The SspH/IpaH family of novel E3 ligases are found in a number of Gram-negative bacteria and are used to target host enzymes for degradation to support pathogenesis. NELs are found in a number of Gram-negative bacteria, such as the mammalian pathogens Salmonella and Shigella and plant pathogens Ensifer fredii and Ralstonia solanacearum. They are composed of an N-terminal secretion motif, a leucine-rich repeat (LRR) domain, and a C-terminal NEL catalytic domain and are structurally conserved across the family. Crystal structures and mechanistic studies of NELs have provided insight into the activities of the two key functional domains: the LRR domain, which is responsible for substrate recognition, and the NEL domain, which can be divided into two subdomains: the C-terminal subdomain containing the E2–Ub binding domain (E2–UbBD) “thumb" and the N-terminal subdomain, which encompasses the catalytic E3 region containing the active site cysteine. Many pathogenic bacteria contain E3 ligases, most of which structurally resemble their eukaryotic counterparts, yet some bacteria, including Salmonella and Shigella, have evolved a new class of E3 ligases, the novel E3 ligase (NEL) family, that have no structural homology to eukaryotic E3s in their catalytic domain but function via an active site cysteine, analogous to HECT or RBR E3 ligases. These catalytic cysteine-containing E3 ligases transfer Ub onto the substrate in a two-step reaction: first, Ub is transferred from the E2–Ub conjugate to form an E3–Ub conjugate in a transthiolation reaction, and subsequently onto lysine residues in the substrate or Ub itself via an aminolysis reaction.

To better understand the mechanism of SspH1 and the apparent differences in activity, we solved the crystal structure of a construct containing the LRR and NEL domains but lacking the first 160 residues, ΔNSspH1 (now referred to as SspH1). The structure was refined at 2.9 Å resolution with one copy in the asymmetric unit and a P622 space group. The structure is elongated with the LRR (residues 161–393) domain extending away from the NEL domain (residues 405–622), which contains the catalytic cysteine (C492) and the α-helices of the E2–UbBD (residues 623–697). It is similar to IpaH9.8 and IpaH3 in an “open" conformation, with the position of the E2–UbBD relative to the catalytic loop in an analogous position to other bacterial E3 ligase structures. The E2–UbBD of SspH1 consists of two long antiparallel α-helices and a small C-terminal helical segment, as also seen in SspH2. In our SspH1 structure, 60 N-terminal residues, those in the LRR–NEL linker and the loop containing the catalytic C492, have a higher B-factor compared with other residues, suggesting more flexibility in these regions. We observed a symmetry-related molecule in our structure of SspH1, where the E2–UbBD of one molecule sits on the top of the LRR domain, close to its substrate binding interface.

> AEYDAVWSKWERDAPAGESPGRAAVVQEMRDCLNNGNPVLNVGASGLTTLPDRLPPHITTLVIPDNNLTSLPELPEGLRELEVSGNLQLTSLPSLPQGLQKLWAYNNWLASLPTLPPGLGDLAVSNNQLTSLPEMPPALRELRVSGNNLTSLPALPSGLQKLWAYNNRLTSLPEMSPGLQELDVSHNQLTRLPQSLTGLSSAARVYLDGNPLSVRTLQALRDIIGHSGIRIHFDMAGPSVPREARALHLAVADWLTSAREGEAAQADRWQAFGLEDNAAAFSLVLDRLRETENFKKDAGFKAQISSWLTQLAEDAALRAKTFAMATEATSTCEDRVTHALHQMNNVQLVHNAEKGEYDNNLQGLVSTGREMFRLATLEQIAREKAGTLALVDDVEVYLAFQNKLKESLELTSVTSEMRFFDVSGVTVSDLQAAELQVKTAENSGFSKWILQWGPLHSVLERKVPERFNALREKQISDYEDTYRKLYDEVLKSSGLVDDTDAERTIGVSAMDSAKKEFLDGLRALVDEVLGSYLTARWRLN> ATAEIKPNKKILIELKVEKKPMGVIVCG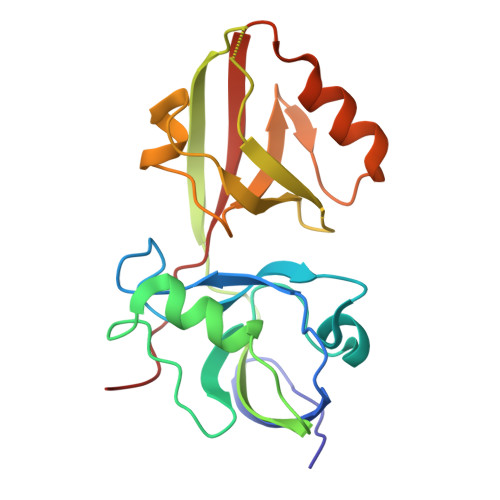GKNNHVTTGCVITHVYPEGQVAADKRLKIFDHICDINGTPIHVGSMTTLKVHQLFHTTYEKAVTLTVFRADPPELEKFNVDLMKKAGKELGLSLSPNEIGCTIADLIQGQYPEIDSKLQRGDIITKFNGDALEGLPFQVCYALFKGANGKVSMEVTRPKPTLRTEA> MLPKELLDVRRAKGRIFPKFADERDYELAEKVIEIFKKGLGKKYGNLMKQARKLENAKNFKKVRGFIRVLENHCIEKSCAFDVDSELEPRKVRMLLFEHGFVTSKKERDRVLEYVARYFSTTPETVERAMYADREEELILTKFRPLTPDNLIKLYNLSLLQTTLFNALRLTFWASDRHKEIFRSIKRL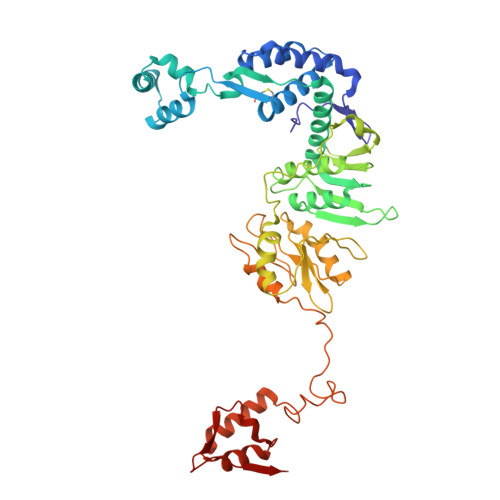GLMYELYEDSGRLMVEVTGAATLLKMTRKYGVSFAKLIPWILRAKNWFIRAEISDFDRLYIMEIDDRIRDLFPDVEERLSYDSTLEEEFARKMQMLGYEVEREPDVVKAGKYAFIPDFAVNLGDKKVYIEIAGFWTDEYLRKKAEKIKSSSIPLILIAREDFGDGGANVKDVILFSRKIPYGEVIKALKRYKPEKKVEGDVVELENFAEVPSEYVIAGKYAVRREIFEEIKREIEVSNPSTLEDIKAILKKYGLGESAIRAFGYRVRWIGLGEAVIERTD> AKTYTLTDYLKNTYRLKLYSLRWISDHEYLYKQENNILVFNAEYGNSSVFLENSTFDEFGHSINDYSISPDGQFILLEYNYVKQWRHSYTASYDIYDLNKRQLITEERIPNNTQWVTWSPVGHKLAYVWNNDIYVKIEPNLPSYRITWTGKEDIIYNGITDWVYEEEVFSAYSALWWSPNGTFLAYAQFNDTEVPLIEYSFYSDESLQYPKTVRVPYPKAGAVNPTVKFFVVNTDSLSSVTNATSIQITAPASMLIGDHYLCDVTWATQERISLQWLRRIQNYSVMDICDYDESSGRWNCLVARQHIEMSTTGWVGRFRPSEPHFTLDGNSFYKIISNEEGYRHICYFQIDKKDCTFITKGTWEVIGIEALTSDYLYYISNEYKGMPGGRNLYKIQLSDYTKVTCLSCELNPERCQYYSVSFSKEAKYYQLRCSGPGLPLYTLHSSVNDKGLRVLEDNSALDKMLQNVQMPSKKLDFIILNETKFWYQMILPPHFDKSKKYPLLLDVYAGPCSQKADTVFRLNWATYLASTENIIVASFDGRGSGYQGDKIMHAINRRLGTFEVEDQIEAARQFSKMGFVDNKRIAIWGWSYGGYVTSMVLGSGSGVFKCGIAVAPVSRWEYYDSVYTERYMGLPTPEDNLDHYRNSTVMSRAENFKQVEYLLIHGTADDNVHFQQSAQISKALVDVGVDFQAM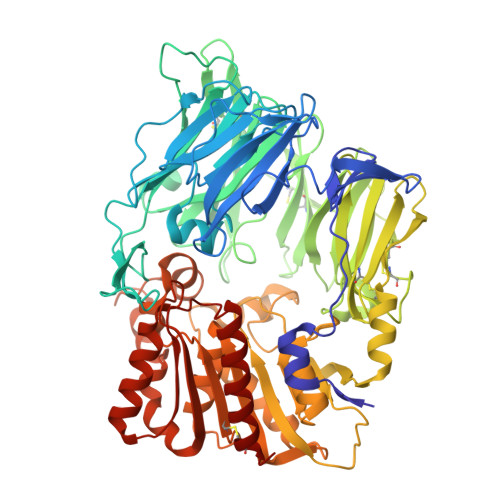WYTDEDHGIASSTAHQHIYTHMSHFIKQCFSL>MAIAQLATEYVFSDFLLKEPTEPKFKGLRLELAVDKMVTCIAVGLPLLLISLAFAQEISIGTQISCFSPSSFSWRQAAFVDSYCWAAVQQKNSLQSESGNLPLWLHKFFPYILLLFAILLYLPPLFWRFAAAPHICSDLKFIMEELDKVYNRAIKAAKSARDLDMRDGACSVPGVTENLGQSLWEVSESHFKYPIVEQYLKTKKNSNNLIIKYISCRLLTLIIILLACIYLGYYFSLSSLSDEFVCSIKSGILRNDSTVPDQFQCKLIAVGIFQLLSVINLVVYVLLAPVVVYTLFVPFRQKTDVLKVYEILPTFDVLHFKSEGYNDLSLYNLFLEENISEVKSYKCLKVLENIKSSGQGIDPMLLLTNLGMIKMDVVDGKTPMSAEMREEQGNQTAELQGMNIDSETKANNGEKNARQRLLDSSCLEWSHPQFEK[7x]

Pannexin 1 (PANX1) plays extensive physiological roles across diverse fields of biology, including cell death, inflammation, cancer progression, and neurological disorders. As suggested by biochemical analysis, PANX1 forms an oligomeric channel for the facilitated diffusion of ions and large molecules across the plasma membrane upon activation. The overall structure of human PANX1 presents a novel heptameric assembly, which is distinct from gap junction channels (connexins and innexins)8,9 and functionally related channels, such as CALHM and LRRC8. Interestingly, the protomer of PANX1 shares a similar fold of four transmembrane helices with the aforementioned channels.

We purified full-length human PANX1 and solved the structure using cryo-EM. Among the classes of 2D particle images, the images representing the top views or bottom views exhibited seven obvious subunits in each detergent micelle. This observation differs from the previously proposed hexameric assembly of PANX1.7 Finally, the map was refined to 3.1 Å resolution. The model we built contained an almost intact extracellular region, transmembrane domain, and partial intracellular region. Three fractions (N-terminal, 1–12; 158–193, between TM2 and TM3; and C-terminal, 355–426) were missing in the final model. Thus, the structure of full-length PANX1 was employed for the following structural analysis due to its clearer density map. As the result shows, the radius of the narrowest constrictive site is ~4.7 Å, which is contributed by W74. I58 from the tail of TM1 forms a larger hydrophobic ring. We discovered a shrink ring formed by residues (T21/E22/P23) in the N-terminus. However, disordered CT tails are missing in the structure of full-length PANX1. Given that the pore is more than 9 Å wide, an open conformation of PANX1 was probably captured.> MAMLSERMLKALNDQLNRELYSAYLYFAMAAYFEDLGLEGFANWMKAQAEEEIGHALRFYNYIYDRNGRVELD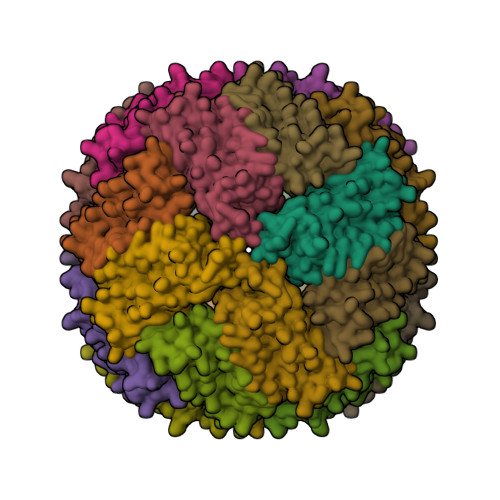EIPKPPKEWESPLKAFEAAYEHEKFISKSIYELAALAEEEKDYSTRAFLEWFINEQVEEEASVKKILDKLKFAKDSPQILFMLDKELSARAPKLPGLLMQGGE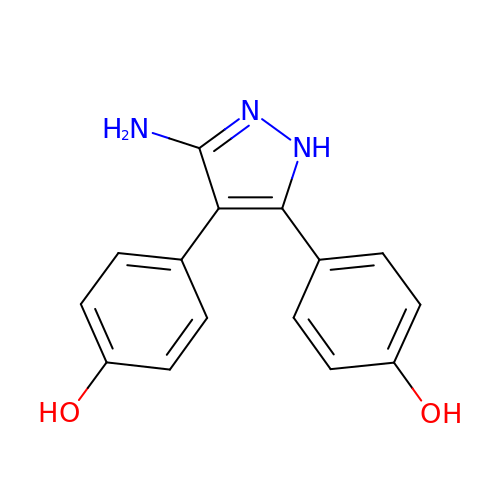4,4'-(3-amino-1H-pyrazole-4,5-diyl)diphenol | C15 H13 N3 O2 | SDULBSMUWSNMKJ-UHFFFAOYSA-N>TSSANEDMPVERILEAELAVEPKTETYVEANMGLNPSSPNDPVTNICQAADKQLFTLVEWAKRIPHFSELPLDDQVILLRAGWNELLIASFSHRSIAVKDGILLATGLHVHRNSAHSAGVGAIFDRVLTELVSKMR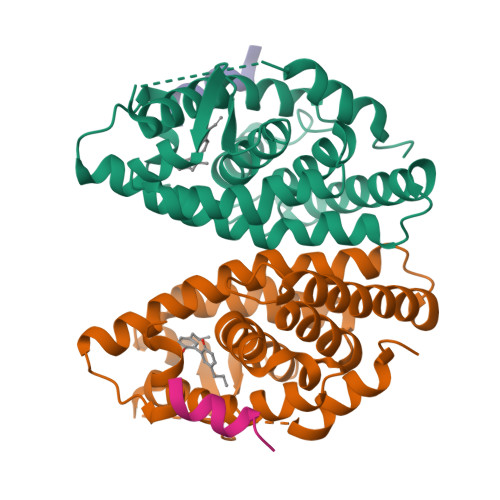DMQMDKTELGCLRAIVLFNPDSKGLSNPAEVEALREKVYASLEAYCKHKYPEQPGRFAKLLLRLPALRSIGLKCLEHLFFFKLIGDTPIDTFLMEMLEAPHQMT[2x];>HKILHRLLQD[2x]>[2x]GSTIEAGIAYPISTGFDPLTSSGASSMAANLHIFEGLVDLHPVTRQPYLALAAKEPEQKDDLTYYISLREGAMFHDGSPVTTEDVVYSFERVLDPAKASLFAQFIPFIASVTALDDNVVEFKLKYPFALFKERLTIIKIVPKHIVEAGQSAFDAKPIGSGPYKFVSATK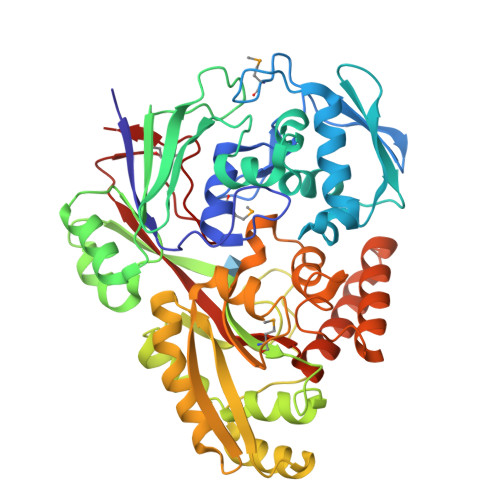DDRIVFEANTVYNGHYPAKVEKMTWFLLSDDAARVTAQESGRVQAIESVPYLDAERLKRKNNVESVQSFGLLFLMFNCEKAPFDNPKVRQALHYALDKQKLIDIVFLGNAKAATSYLQDTHPDYVKASSQYDYDKAKAEKLLAEAGITNLTFQLLATDHAWVKECAPLILESWNALSVVKVTLQHLQSGALYSAHVDKGAYEVVIAPGDPSVFGNDLDLLLSWWYRGDVWPKRRFRWANTAEYHEVQKLLDEAIKNPAGSKVAWQKAINIIAEQVPLYPIIHRKLPTAWNTKKLTDFQPLPTTGLSFLGVGRT> MADKELKFLVVDDFSTMRRIVRNLLKELGFNNVEEAEDGVDALNKLQAGGYGFVISDWNMPNMDGLELLKTIRADGAMSALPVLMVTAEAKKENIIAAAQAGASGYVVKPFTAATLEEKLNKIFEKLGM;> MMQPSIKPADEHSAGDIIARIGSLTRMLRDS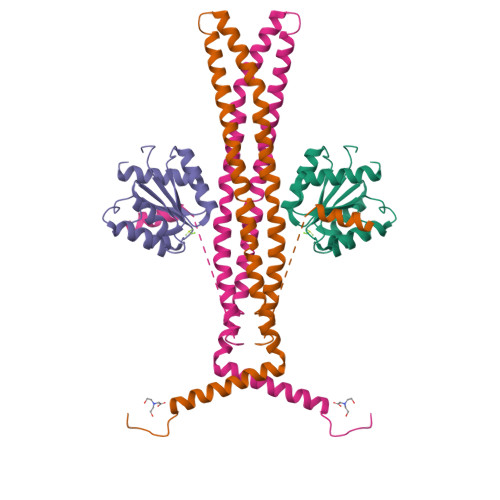LRELGLDQAIAEAAEAIPDARDRLYYVVQMTAQAAERALNSVEASQPHQDQMEKSAKALTQRWDDWFADPIDLADARELVTDTRQFLADVPAHTSFTNAQLLKIMMAQDFQDLTGQVIKRMMDVIQEIERQLLMVLLENIPEQESRPKRENQSLLNGPQVDTSKAGVVASQDQVDDLLDSLGF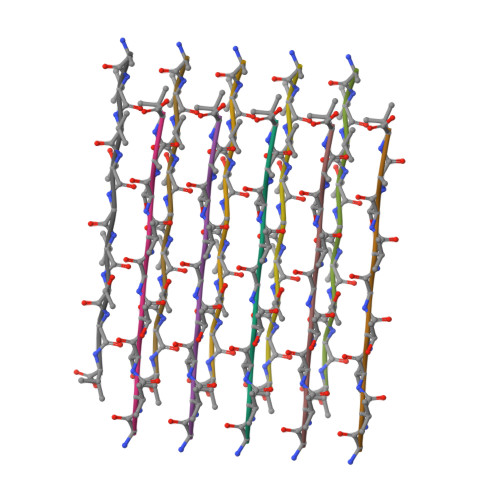> AVVTGVTAV> ETSYTLNEVVPLKEFVPEWVRI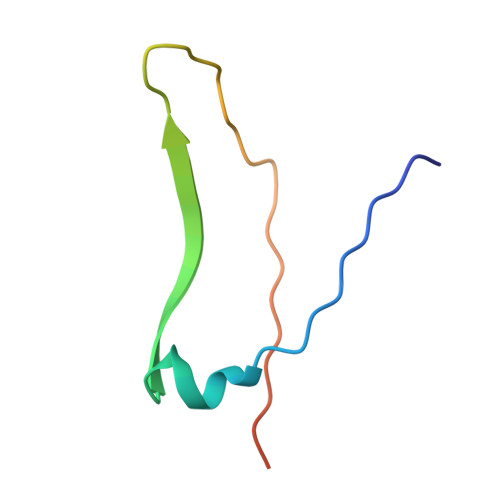GFSATTGAEFAAHEVLSWYFHSELAGTSSS>[3x]TGCDEMVHADSKLVSCR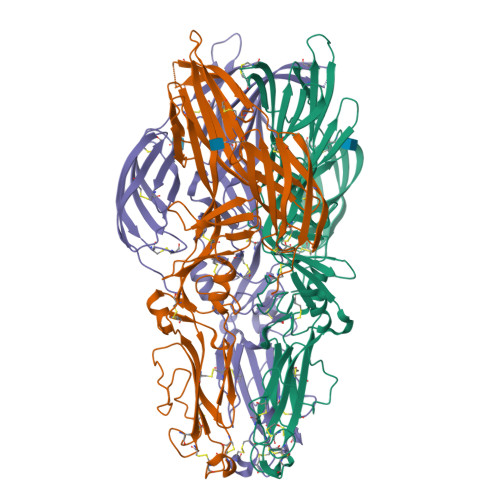QGSGNMKECVTTGRALLPAVNPGQEACLHFTAPGSPDSKCLKIKVKRINLKCKKSSSYFVPDARSRCTSVRRCRWAGDCQSGCPPHFTSNSFSDDWAGKMDRAGLGFSGCSDGCGGAACGCFNAAPSCIFWRKWVENPHGIIWKVSPCAAWVPSAVIELTMPSGEVRTFHPMSGIPTQVFKGVSVTYLGSDMEVSGLTDLCEIEELKSKKLALAPCNQAGMGVVGKVGEIQCSSEESARTIKKDGCIWNADLVGIELRVDDAVCYSKITSVEAVANYSAIPTTIGGLRFERSHDSQGKISGSPLDITAIRGSFSVNYRGLRLSLSEITATCTGEVTNVSGCYSCMTGAKVSIKLHSSKNSTAHVRCKGDETAFSVLEGVHSYTVSLSFDHAVVDEQCQLNCGGHESQVTLKGNLIFLDVGTKHHHHHH(4S,4a'S,10a'R)-2-amino-8'-(2-fluoropyridin-3-yl)-1-methyl-3',4',4a',10a'-tetrahydro-2'H-spiro[imidazole-4,10'-pyrano[3,2-b]chromen]-5(1H)-one 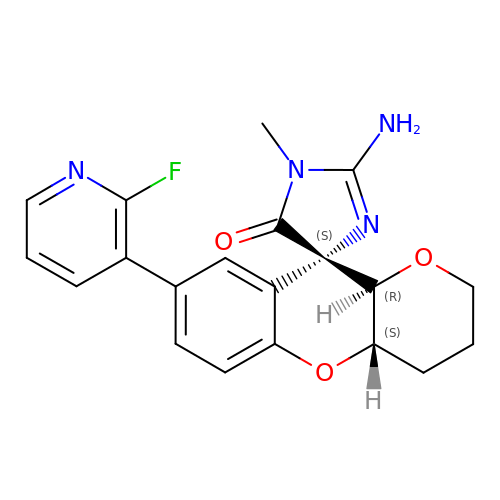| C20 H19 F N4 O3 | GZRDWAATBYKNGI-FTRWYGJKSA-N N-[(1S)-1-benzyl-2-[(6-chloro-2-oxo-1H-quinolin-4-yl)methylamino]-2-oxo-ethyl]-4-hydroxy-2-oxo-1H-quinoline-6-carbo | C29 H23 Cl N4 O5 | 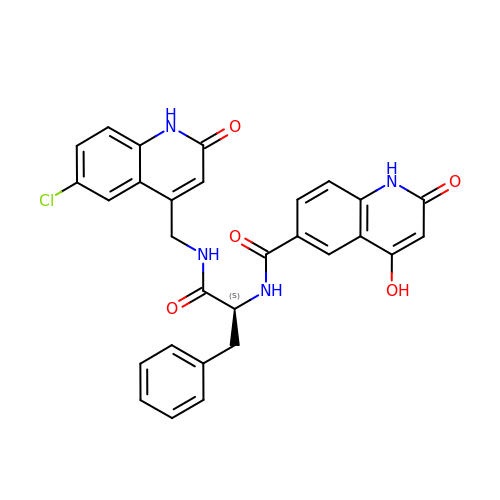DNDMLXSODUEUMP-DEOSSOPVSA-N>[4x]MQEVTLTLHQFLPA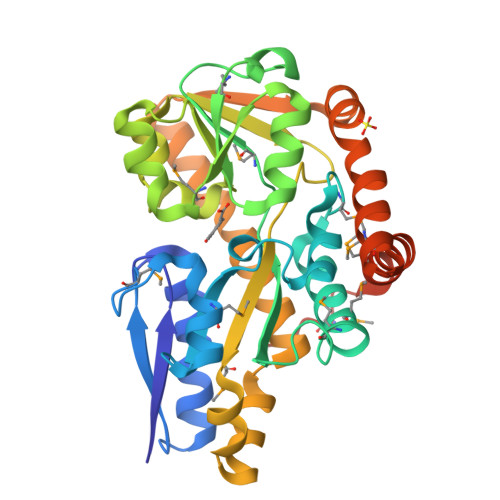QANVPKDVLDVWADNVEEASDGRIEIERYPSMQLGGTPPELMDQAIDGIADIVWTVVGYTPGRYPSTEVFELPFMVSDARAASYAYWKMFEEHMKDGEFADVKILGTWVHGPGMFHTNKPVAVPSDLEGMKIRGGSRLVNDLLTRVGAEPIGMPVPAISEALSKGVIDGTTIPWEVTSALKVPELVGNHTEFDGPALYNLTFVLAMNKDAYESLPEDLQEVIDSQSGLAFSIFAGGTQADADGPARQIAVDRGNNIVTVSQEDAKAWDALVNPIYETWVAEMNDKGIDGQALIDEAKSLMEEYDPSMDTYGKAAALEHHHHHH> SEQTEVLKPRTLADLIRILHQLFAGDEVNVEEVQAIMEAYESDPTEWAMYAKFDQYRYTRNLVDQGNGKFNLMILC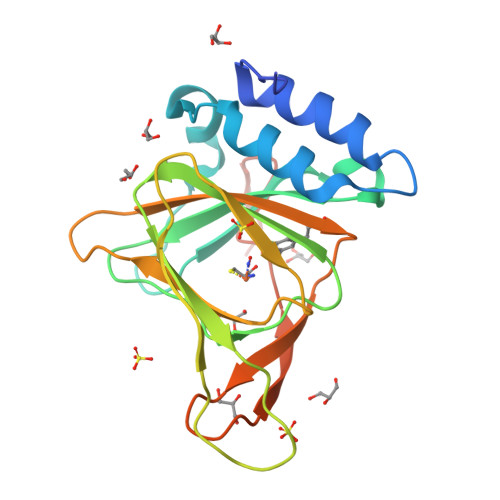WGEGHGSSIHDHTNSHCFLKMLQGNLKETLFAWPDKKSNEMVKKSERVLRENQCAYINDSVGLHRVENISHTEPAVSLHLXSPPFDTCHAFDQRTGHKNKVTMTFHSKFGIRTPNATSGSLENN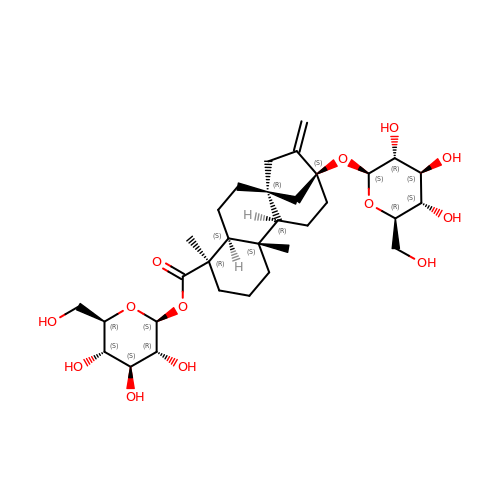1-O-[(8alpha,9beta,10alpha,13alpha)-13-(beta-D-glucopyranosyloxy)-18-oxokaur-16-en-18-yl]-beta-D-glucopyranose | C32 H50 O13 | YWPVROCHNBYFTP-OSHKXICASA-N> PQYQTWEEFSRAAEKLYLADPMKARVVLKYRHSDGNLCVKVTDDLVCLVYKTDQAQDVKKIEKFHSQLMRLMVAKEARNVTMETE;> VLLESEQFLTELTRLFQKCRTSGSVYITLKKYDGRTKPIPKKG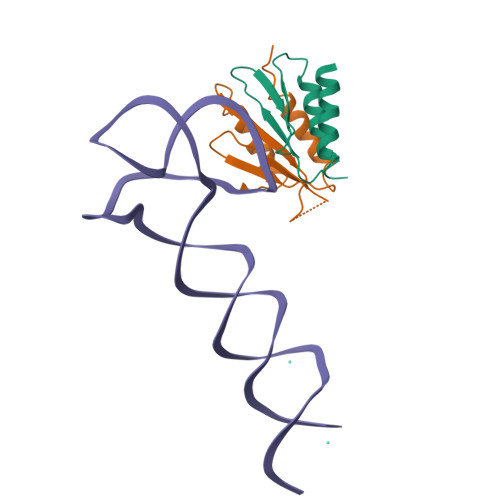TVEGFEPADNKCLLRATDGKKKISTVVSSKEVNKFQMAYSNLLRANMDGLKKRDKKNKTKKTK> PRVVPDQRSKFENEEFFRKLSRECEIKYTGFRDRPHEERQARFQNACRDGRSEIAFVATGTNLSLQFFPASWQ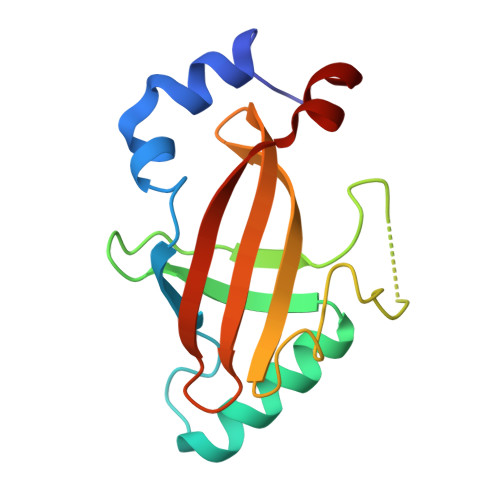GEQRQTPSREYVDLEREAGKVYLKAPMILNGVCVIWKGWIDLQRLDGMGCLEFDEERAQQE(3-fluoroazetidin-1-yl){1-[4-(4-fluorophenyl)pyrimidin-5-yl]piperidin-4-yl}methanone 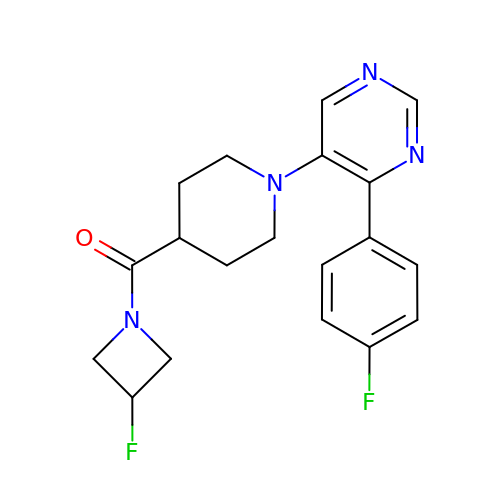| C19 H20 F2 N4 O | UTHXOPCOQREWLE-UHFFFAOYSA-N>GSPCPGACVCYNEPKVTTSCPQQGLQAVPTGIPASSQRIFLHGNRISHVPAASFQSCRNLTILWLHSNALARIDAAAFTGLTLLEQLDLSDNAQLHVVDPTTFHGLGHLHTLHLDRCG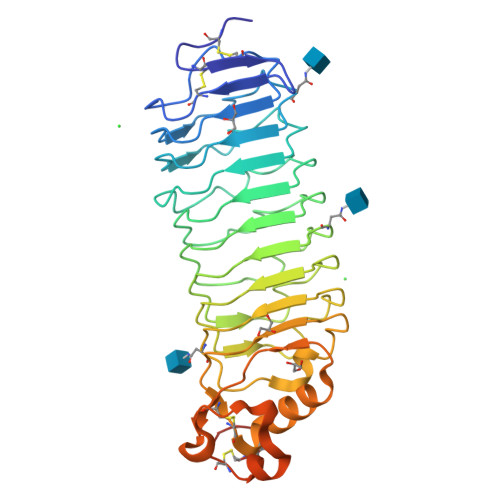LRELGPGLFRGLAALQYLYLQDNNLQALPDNTFRDLGNLTHLFLHGNRIPSVPEHAFRGLHSLDRLLLHQNHVARVHPHAFRDLGRLMTLYLFANNLSMLPAEVLMPLRSLQYLRLNDNPWVCDCRARPLWAWLQKFRGSSSEVPCNLPQRLADRDLKRLAASDLEGCAVASGPFRPIQTSQLTDEELLSLPKCCQAAAHHHHHH[2x]> STLQFKVGPPFELVRD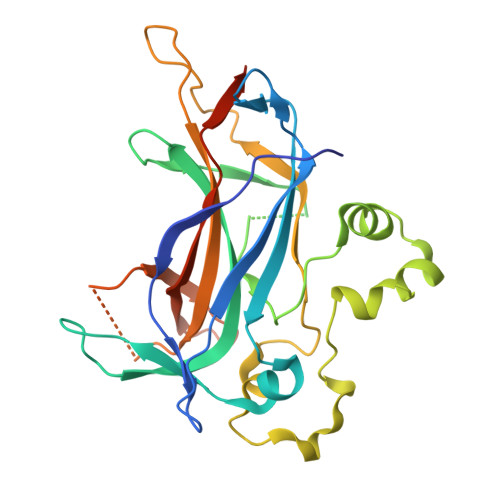YCPVVESHTGRTLDLRIIPRIDRGFDHIDEEWVGYKRSYFTLVSTFETANCDLDTFLKSSFDLLVEDSSVEGRLRVQYFAIKIKAKNDDDDTEINLVQHTAKRDKGPQFCPSVCPLVPSPLPKHQIIREASNVRNITKMKKYDSTFYLHRDHVNYEEYGVDSLLFSYPEDSIQKVARYERVQFASSISVKKPSQQNKHFSLHVILGAVVDPDTFHGENPGIPYDELALKNGSKGMFVYLQEMKTPPLIIRGRSPSNYASSQRITVR Type IV pili are found in many Gram-negative bacteria as well as in some Gram-positive bacteria and archaea, where they function in numerous cellular processes including adhesion, DNA transfer and virulence. Furthermore, in the metal reducing bacteria Shewanella oneidensis and Geobacter sulfurreducens type IV pili have been implicated in extracellular electron transport (EET) pathways. PilBac1ΔN consists of one long N-terminal α-helix packed against 4 antiparallel β-strands resembling the core fold of type IV pilins. Interestingly, our PilBac1 crystal structure reveals two unusual features compared to other type IVa pilins: an unusual position of the disulfide bridge and a straight α-helical section, which usually exhibits a pronounced kink.

The potential nanowire type IV pilin PilBac1 from S. oneidensis was characterized by a combination of complementary structural methods and the atomic structure was determined at a resolution of 1.67 Å by X-ray crystallography. To obtain a soluble version of PilBac1, a construct was designed that lacks the N-terminal 35 residues including the signal peptide and the transmembrane α-helix. A high resolution data set was collected on another crystal and data were processed in the high symmetry space group I222 to a resolution of 1.67 Å using the CC1/2 value as a cut-off. The model obtained from S-SAD was then used as a search model in molecular replacement for this data set, and all residues were modelled into clear electron density with no apparent ambiguities. The crystal form had a large solvent content (62%) yielding a high optical resolution and favorable data-to-parameter ratio at 1.67 Å resolution. PilBac1ΔN was crystallized as a parallel dimer in the asymmetric unit in which the interface is formed by interactions between 15 and 20 residues in the α-helix from monomers A and B, respectively (forming a non-proper dimer with a screw-axis) (R.M.S.D. of 0.309 Å based on 79 out of a total of 89 Cαs). A: Sodium ion binding site in chain B. The Na+ ion is coordinated by the backbone oxygens of Leu36 and Phe44, as well as the side chain oxygen of Asn38 and three water molecules. Interestingly, this sodium ion was not observed in chain A due to a slight distortion of the ion binding site compared to chain B. The backbone of Leu36 is further away from the binding site increasing the distance from 2.6 to 3.7 Å. Interestingly, PilBac1 possesses a helix breaking proline at position 22, but a helix breaking residue is missing at position 42. Therefore, kink 2 is missing in PilBac1 and the α-helix in the structure of PilBac1ΔN is straight.

>[2x]GKQGRRFDAQQYLVTSAQALERHYSRNGLYPASQSLANSPYYSFSYTPTADKFGFSLKAVPTNRQSDPCGTLSLDHKGVRVPATNCWSH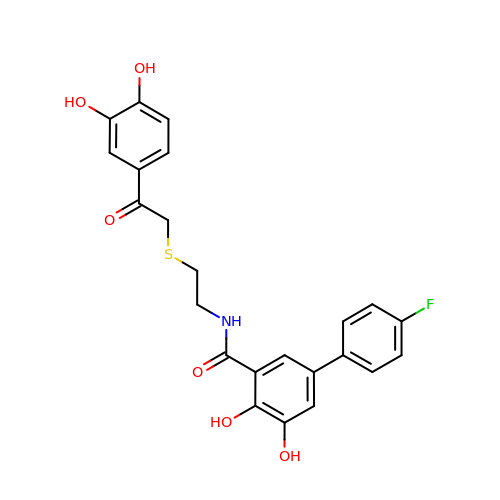N-[2-[2-(3,4-dihydroxyphenyl)-2-oxoethyl]sulfanylethyl]-5-(4-fluorophenyl)-2,3-dihydroxybenzamide | C23 H20 F N O6 S | HAURVZGCSFOKBL-UHFFFAOYSA-N> MVNISDFFGKNKKSVRSSTSRPTRQVGSSKPEVIDLDTESDQESTNKTPKKMPVSNVIDVSETPEGEKKLPLPAKRKASSPTVKPASSKKTKPSSKSSDSASNITAQDVLDKIPSLDLSNVHVKENAKFDFKSANSNADPDEIVSEIGSFPEGKPNCLLGLTIVFTGVLPTLERGASEALAKRYGARVTKSISSKTSVVVLGDEAGPKKLEKIKQLKIKAIDEEGFKQLIAGMPAEGGDGEAAEKARRKLEEQHNIATKEAELLVKKEEERSKKLAATRVSGGHLERDNVVREEDKLWTVKYAPTNLQQVCGNKGSVMKLKNWLANWENSKKNSFKHAGKDGSGVFRAAMLYGPPGIGKTTAAH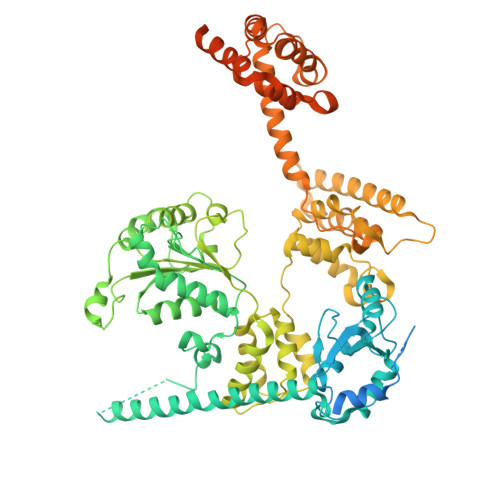LVAQELGYDILEQNASDVRSKTLLNAGVKNALDNMSVVGYFKHNEEAQNLNGKHFVIIMDEVDGMSGGDRGGVGQLAQFCRKTSTPLILICNERNLPKMRPFDRVCLDIQFRRPDANSIKSRLMTIAIREKFKLDPNVIDRLIQTTRGDIRQVINLLSTISTTTKTINHENINEISKAWEKNIALKPFDIAHKMLDGQIYSDIGSRNFTLNDKIALYFDDFDFTPLMIQENYLSTRPSVLKPGQSHLEAVAEAANCISLGDIVEKKIRSSEQLWSLLPLHAVLSSVYPASKVAGHMAGRINFTAWLGQNSKSAKYYRLLQEIHYHTRLGTSTDKIGLRLDYLPTFRKRLLDPFLKQGADAISSVIEVMDDYYLTKEDWDSIMEFFVGPDVTTAIIKKIPATVKSGFTRKYNSMTHPVAIYRTGSTIGGGGVGTSTSTPDFEDVVDADDNPVPADDEETQDSSTDLKKDKLIKQKAKPTKRKTATSKPGGSKKRKTKA INOSITOL-(1,3,4,5,6)-PENTAKISPHOSPHATE | C6 H17 O21 P5 | 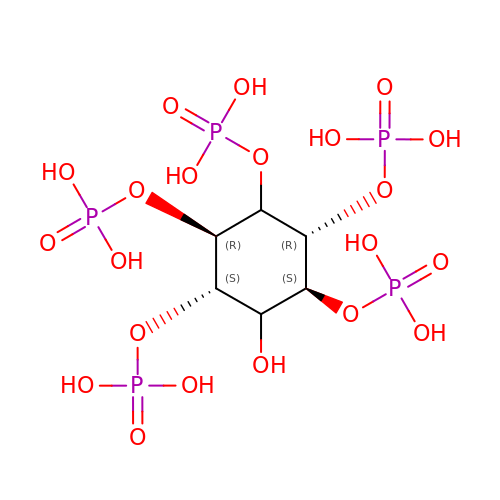CTPQAXVNYGZUAJ-ADOSBGCESA-N> XLAA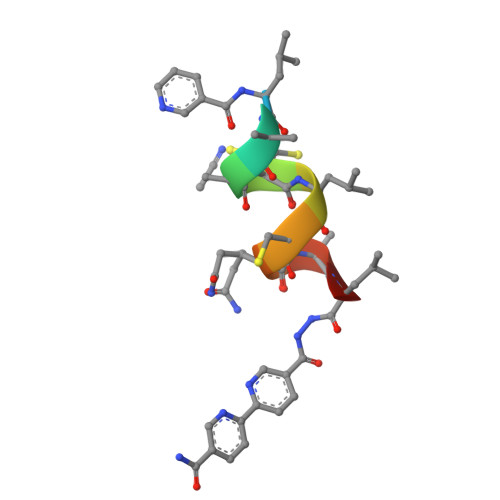CLCQALX>GGCTCGGCGG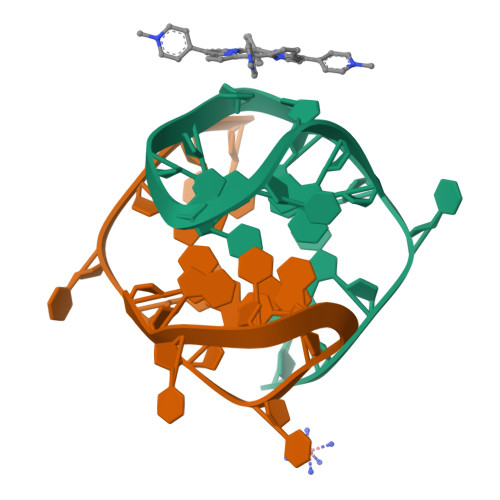CGGA[2x]> SLGLQDFDLLRVIGRGSYAKVLLVRLKKTDRIYAMKVVKKELVNDDEDIDWVQTEKHVFEQASNHPFLV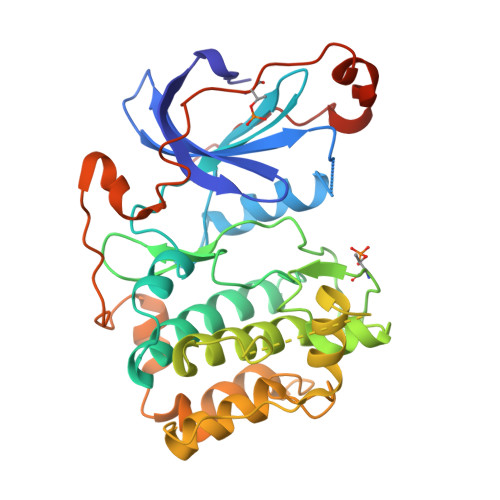GLHSCFQTESRLFFVIEYVNGGDLMFHMQRQRKLPEEHARFYSAEISLALNYLHERGIIYRDLKLDNVLLDSEGHIKLTDYGMCKEGLRPGDTTSTFCGTPNYIAPEILRGEDYGFSVDWWALGVLMFEMMAGRSPFDIVGSSDNPDQNTEDYLFQVILEKQIRIPRSLSVKAASVLKSFLNKDPKERLGCHPQTGFADIQGHPFFRNVDWDMMEQKQVVPPFKPNISGEFGLDNFDSQFTNEPVQLTPDDDDIVRKIDQSEFEGFEYINPLLMSAEECV2,4-DIAMINO-6-[N-(2',5'-DIMETHOXYBENZYL)-N-METHYLAMINO]QUINAZOLINE 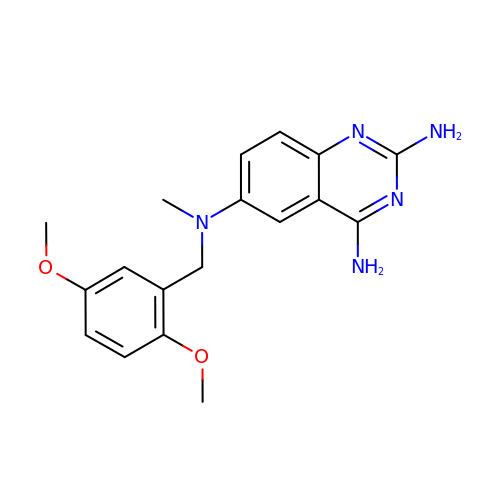| C18 H21 N5 O2 | YBJANOUTWRTBDK-UHFFFAOYSA-N>[2x]MAHHHHHHMPFDVIWMEVEMAKMRVGIVFGGKSAEHEVSLQSAKNIVEAIDKSRFDVVLLGIDKQGLWHINDAGNYLLNAQDPARIALRPSTVTLAQIPGREAQQLINAESGQPLAAIDVIFPIVHGTLGEDGSLQGMLRMANLPFVGSDVLGSAACMDKDVTKRLLRDAGLAVA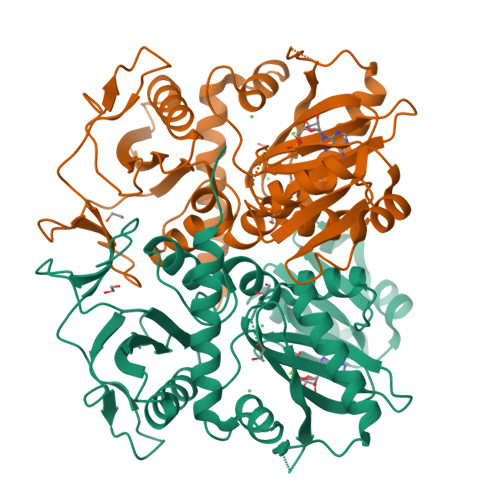PFITLTRANRAQFSFADVEAKLGLPLFVKPANQGSSVGVSKVKNEEQYHQAVALAFEFDHKVVVEQGIKGREIECAVLGNDHPQASTCGEIVLNSEFYAYDTKYIDDQGAQVVVPAAIAPEINDKIRAIAVQAYQTLGCSGMARVDVFLTADNEVVINEINTLPGFTNISMYPKLWQASGLDYTSLITRLIELALERHAADRALKTSMN> KMAR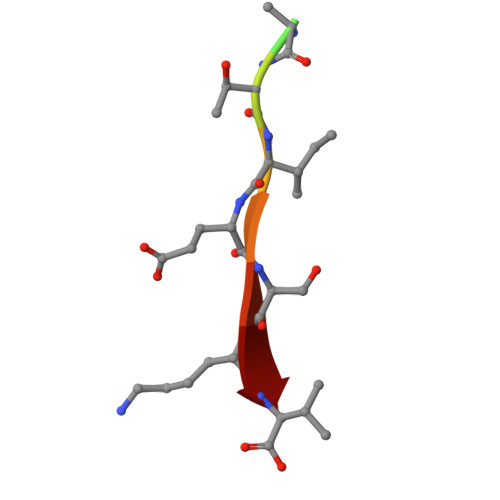TIESKV> KHYITYRINNYTPDMNREDVDYAIRKAFQVWSNVTPLKFSKINTGMADILVVFARGAHGDDHAFDGKGGILAHAFGPGSGIGGDAHFDE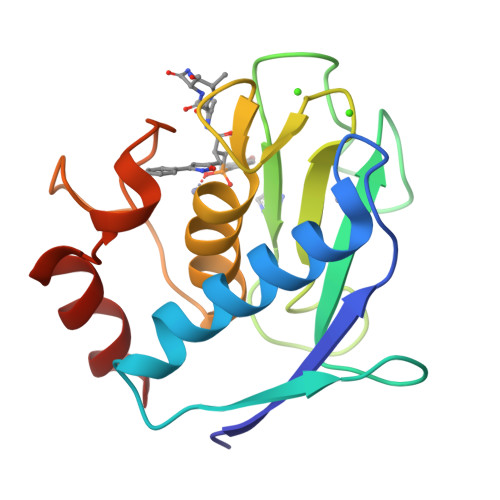DEFWTTHSGGTNLFLTAVHEIGHSLGLGHSSDPKAVMFPTYKYVDINTFRLSADDIRGIQSLY>[5x]MGLFLEDLAVGDRFDSARHRVEAAAIKAFAGEFDPQPFHLDEEAARHSLFGGLAASGWHTAAITMR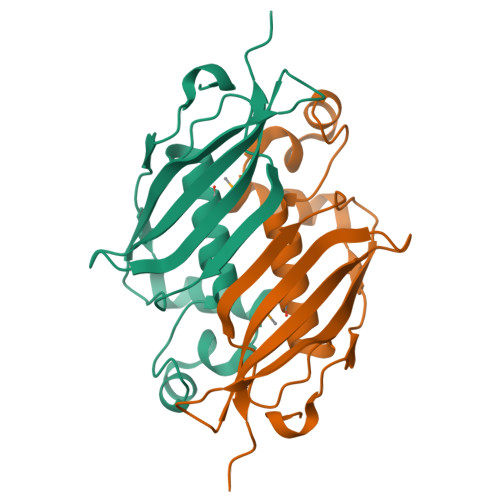LLVTSGLPLAQGIIGAGTELSWPNPTRPGDELHVETTVLAITPSKSRPDRAIVTCQSDTLNQRGEVVQRSTAKVVVFRRPLEHHHHHH> GSMGDTKEQRILNHVLQHAEPGNAQSVLEAIDTYCEQKEWAMNVGDKKGKIVDAVIQEHQPSVLLELGAYCGYSAVRMARLLSPGARLITIEINPDCAAITQRMVDFAGVKDKVTLVVGASQDIIPQLKKKYDVDTLDMVFLDHWKDRYLPDTLLLEECGLLRKGTVLLADNVICPGAPDFLAH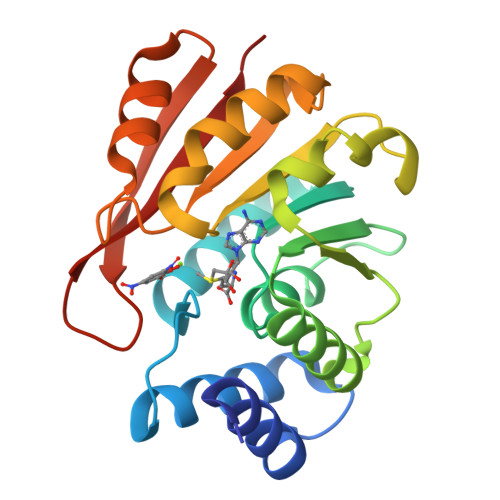VRGSSCFECTHYQSFLEYREVVDGLEKAIYKG>[2x]SIAAKEEGVSLEKR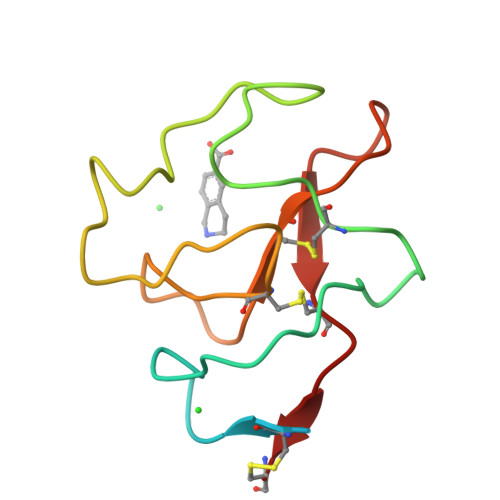SIARSDCYHGDGQSYRGSFSTTVTGRTCQSWSSMTPHWHQRTTEYYPNGGLTRNYCRNPDAEIRPWCYTMDPSVRWEYCALTQC> PLGSKDNRLLYPKTKIDWGPGENHICLKTPFKNFYVIELFHQAPTFDKTIPLFISDINNSPNLYGIYNYIADHLRHVVLVNNYPVNQINIFGKIVYEQYKEKEFNGVEESYVILVISDFIGIDSKIRVRLSQEQFKEVGLTLDKKNYGKIVELEGEIYN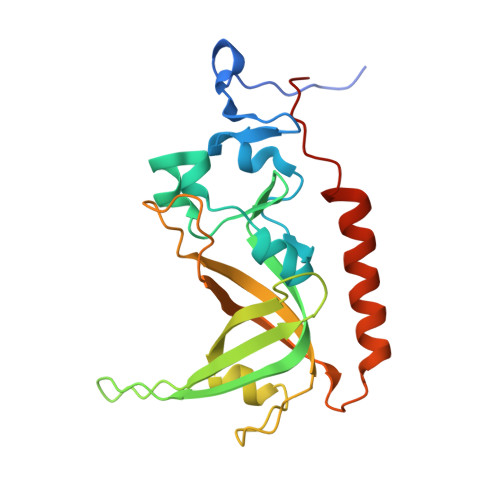WYDSINVSKKPDRELKVSKITVLSHRPDGLHFEFEQWKKRMEFRKNNLVEPWVFIPTPQRE The core of the glideosome consists of an atypical class XIV myosin A (PfMyoA) and a divergent actin (PfAct1). PfMyoA is a short myosin with a conserved globular motor domain and a lever arm that binds two light chains: an essential light chain (PfELC) and myosin tail interacting protein (MTIP). PfMyoA is a critical molecule in the parasite life-cycle because it powers the fast motility (~2 µm.s−1) required during motile sporozoite stages, and is essential for providing the force (up to 40 pN) needed for non-motile merozoites to invade erythrocytes. Here, we present the X-ray structures of full-length (FL) PfMyoA complexed to PfELC and MTIP in two states of the motor cycle.

We determined the crystal structures of FL PfMyoA with two light chains bound (PfMyoA/PfELC/MTIP-Δn) in the post-rigor (PfMyoA•FL-PR) and in the pre-powerstroke (PfMyoA•FL-PPS) states at 2.5 Å and 3.9 Å resolution, respectively. In the PPS states, crystallized with ADP and Pi analogs, however, the converter orientation is less primed by ~30° in the MD structure compared with that found in the FL structure (Robert-Paganin et al., 2019). SAXS experiments validated that the PPS of PfMyoA adopts the more primed orientation in solution. Notably, the lever arm is more primed in the PPS state of PfMyoA compared with that of conventional myosins, leading to a larger powerstroke than most myosins. We describe below the converter/PfELC interface (interface A) seen in the PfMyoA•FL-PPS crystal structure, which is similar to the solution structure. In PfMyoA, a more rigid interface forms because it involves mainly hydrophobic contributions from the α5*, α5’*, and α6 helices whose conformations are stabilized by W777. The atypical priming of the PfMyoA lever arm in the PPS state results from several interactions between the lever arm and the motor domain that are not present in conventional myosins. Conformational changes at the end of the SH1 helix are required to allow an additional Converter rotation so that it can reach the PfMyoA motor domain surface with which it interacts. These interactions involve two interfaces: interactions of PfELC with Loop-1 and the β-bulge and a specific interface between the Converter and the N-terminal subdomain (N-term). Interestingly, interactions between PfELC, loop-1 and the β-bulge are highly labile during molecular dynamics, but the interface between the Converter and the N-term subdomain is highly stable and maintained throughout the time course. We conclude that the priming seen in the PfMyoA•FL-PPS crystal structure is stable, and that the PfMyoA lever arm is more rigid than in conventional myosins.

>MAVTNEEIKTASKIVRRVSNVEAFDKSGSVFKGYQIWTDISPTIENDPNIMFVKCVVQQGSKKEKLTVVQIDPPGTGTPYDIDPTHAWNCNSQVDPMSFGDIGLLNHTNIPCVLDFLKHRYLKNQIYTTAVPLIVAINPYKDLGNTTNEWIRRYRDTADHTKLPPHVFTCAREALSNLHGVNKSQTIIVSGESGAGKTEATKQIMRYFASSKSGNMDLRIQTAIMAANPVLEAFGNAKTIRNNNSSRFGRFMQLVISHEGGIRYGSVVAFLLEKSRIITQDDNERSYHIFYQFLKGANSTMKSKFGLKGVTEYKLLNPNSTEVSGVDDVKDFEEVIESLKNMELSESDIEVIFSIVAGILTLGNVRLIEKQEAGLSDAAAIMDEDMGVFNKACELMYLDPELIKREILIKVTVAGGTKIEGRWNKNDAEVLKSSLCKAMYEKLFLWIIRHLNSRIEPEGGFKTFMGMLDIFGFEVFKNNSLEQLFINITNEMLQKNFVDIVFERESKLYKDEGISTAELKYTSNKEVINVLCEKGKSVLSYLEDQCLAPGGTDEKFVSSCATNLKENNKFTPAKVASNKNFIIQHTIGPIQYCAESFLLKNKDVLRGDLVEVIKDSPNPIVQQLFEGQVIEKGKIAKGSLIGSQFLNQLTSLMNLINSTEPHFIRCIKPNENKKPLEWCEPKILIQLHALSILEALVLRQLGYSYRRTFEEFLYQYKFVDIAAAEDSSVENQNKCVNILKLSGLSESMYKIGKSMVFLKQEGAKILTKIQREKLVEWENCVSVIEAAILKHKYKQKVNKNIPSLLRVQAHIRKKMVAQ[2x];>[2x]MKQECNVCYFNLPDPESTLGPYDNELNYFTWGPGFEYEPEPQRKPLSIEESFENSEESEESVADIQQLEEKVDESDVRIYFNEKSSGGKISIDNASYNARKLGLAPSSIDEKKIKELYGDNLTYEQYLEYLSICVHDKDNVEELIKMFAHFDNNCTGYLTKSQMKNILTTWGDALTDQEAIDALNAFSSEDNIDYKLFCEDILQ;> MASDMEEKFREAFILFSSCSDHIEMYKFFELMNSFGIILTNDEKAALPNDINMDYWLNFAKKHYNYEQPFKHINNVNEQNTNVQIKIDNFLGIMKALDTRLTESDLNILLQITNPENKTTLNLKTVSQKLTESI;> MASDMEEKFREAFILFSSCSDHIEMYKFFELMNSFGIILTNDEKAALPNDINMDYWLNFAKKHYNYEQPFKHINNVNEQNTNVQIKIDNFLGIMKALDTRLTESDLNILLQITNPENKSTLNLKTVSQKLTESI5-[4-[3-[[2-[(1~{S})-1-oxidanylethyl]imidazol-1-yl]methyl]-1,2-oxazol-5-yl]phenyl]pent-4-yn-1-ol 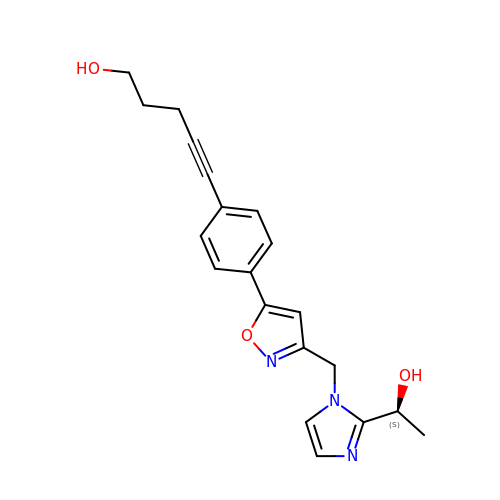| C20 H21 N3 O3 | LYWGLMYUHVPQCZ-HNNXBMFYSA-N>GSEEVVQDAPLENNELNAEIDLQKTIQEEYKLWKQNVPFLYDLVITHALEWPSLTIQWLPDKKTIPGTDYSIQRLILGTHTSGNDQNYLQIASVQLPNFDEDTTEFTPSTIRRAQATGSYTIEISQKIPHDGDVNRARYMPQKPEIIATMGEGGNAYIFDTTCHDALTTGEALPQAVLKGHTAEGFGLCWNPNLPGNLATGAEDQVICLWDVQTQSFTSSETKVISPIAKYHRHTDIVNDVQFHPQHEALLASVSDDCTLQIHDTRLNPEEEAPKVIQAHSKAINAVAINPFNDYLLATASADKTVALWDLRNPYQRLHTLEGHEDEVYGLEWSPHDEPILASSSTDRRVCIWDLEKIGEEQTPEDAEDGSPELLFMHGGHTNRISEFSWCPNERWVVGSLADDNILQIWSPSRVIWGRDHVQVSPRDLE[2x];>[2x]PRVYETELLVLRFREFGVKDNHNHPINLHSLRSKSLIRAQGKKLDLHNRVFLRRNV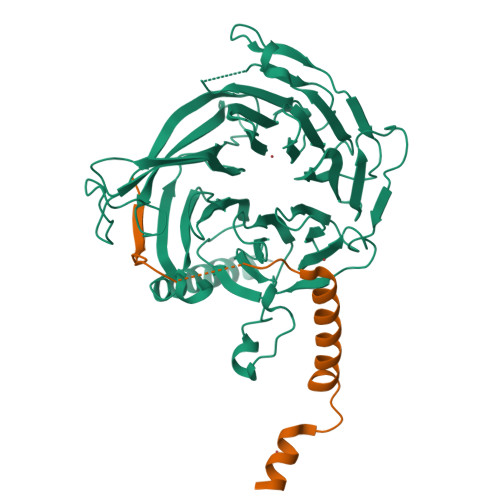RAVKM The BisI family of restriction endonucleases is unique in requiring multiple methylated or hydroxymethylated cytosine residues within a short recognition sequence (GCNGC), and in cleaving directly within this sequence, rather than at a distance. We present the crystal structures of NhoI and Eco15I_Ntd (N-terminal catalytic domain of Eco15I) in the absence of DNA and in specific complexes with fully methylated GCNGC containing dsDNA. Both proteins are homodimeric, with each domain involved in target sequence recognition and catalysis. The crystal structures show that the modified cytosine bases are recognized in the context of double-stranded DNA, without base flipping.

Crystals grown in the absence of DNA contained either an NhoI dimer, or two Eco15I_Ntd dimers in the asymmetric unit. In the NhoI crystal structure without DNA, the dimer adopts a more open conformation overall, primarily due to a different main chain conformation immediately downstream of the dimerization helix α0. However, the hairpin of β-stands β7 and β8 is much better ordered, likely because of crystal contacts to adjacent molecules. Together, the data suggest that NhoI and Eco15I_Ntd can latch onto DNA thanks to an opening of the DNA binding cleft, and due to flexibility of the β-hairpin that closes the DNA binding cleft at the top.

>[2x]GSMSRPPSYAGDMNLENLTTRELLAVSRASLRELKRRGVIRSGNAPAGDYAELLVQRATDGELANASQKSWDIRTTEGDRLQVKARVITDEHANGERQLSTIRSWDFDAAVIVLFDDNFRVWRAARVPAAIMKEAAYYSQHVRGYTVYAKDALLNHSEVEDWTEQLRSVEQ> MARPDDEEGAAVAPGHPLAKGYLPLPRGAPVGKESVELQNGPKAGTFPVNGAPRDSLAAASGVLGGPQTPLAPEEETQARLLPAGAGAETPGAESSPLPLTALSPRRFVVLLIFSLYSLVNAFQWIQYSIISNVFEGFYGVTLLHIDWLSMVYMLAYVPLIFPATWLLDTRGLRLTALLGSGLNCLGAWIKCGSVQQHLFWVTMLGQCLCSVAQVFILGLPSRIASVWFGPKEVSTACATAVLGNQLGTAVGFLLPPVLVPNTQNDTNLLACNISTMFYGTSAVATLLFILTAIAFKEKPRYPPSQAQAALQDSPPEEYSYKKSIRNLFKNIPFVLLLITYGIMTGAFYSVSTLLNQMILTYYEGEEVNAGRIGLTLVVAGMVGSILCGLWLDYTKTYKQTTLIVYILSFIGMVIFTFTLDLRYIIIVFVTGGVLGFFMTGYLPLGFEFAVEITYPESEGTSSGLLNASAQIFGILFTLAQGKLTSDYGPKAGNIFLCVWMFIGIILTALIKSDLRRHNI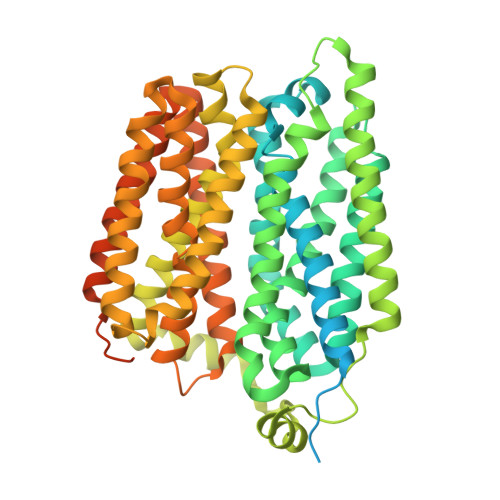NIGITNVDVKAIPADSPTDQEPKTVMLSKQSESAIDYKDDDDK PTERINE | C6 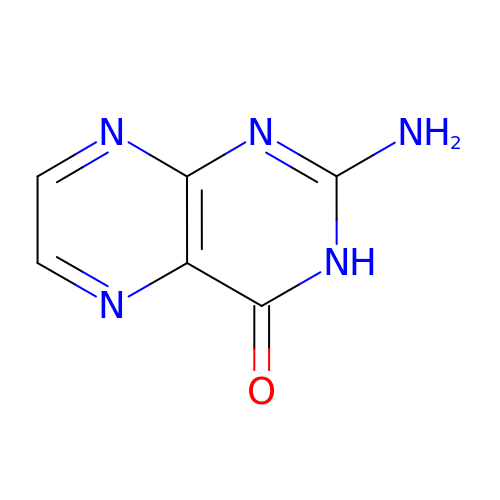H5 N5 O | HNXQXTQTPAJEJL-UHFFFAOYSA-N> MQSSSALTFSPESRQQSGAKMIESQNILNLSPSEKERLSQQQIVFNEVEKDQLHSKANFPLLKNAKGMVIKYDPKVIELKKVGDTVKFQMLEYGI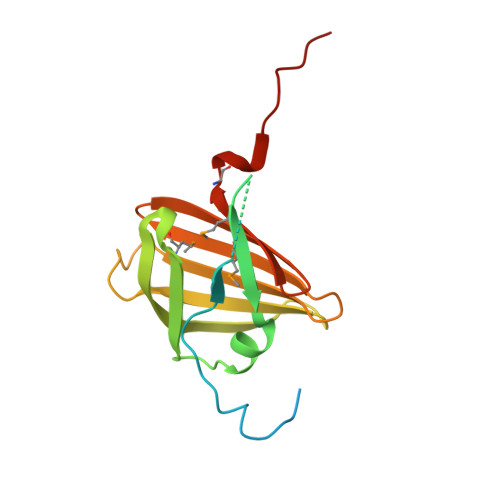NRTGKIVEIEPVDQDIVRWTGRFDQGDPNQNFFTITQSQKDHYTIMQIFTEKGNYSAEIKDGVGLVQTMDEGVTDQELHHDHP> MADYKDDDDKGTDYKDDDDKLEVLFQGPMSLRIDVDTNFPECVVDAGKVTLGTQQRQEMDPRLREKQNEIILRAVCALLNSGGGIIKAEIENKGYNYERHGVGLDVPPIFRSHLDKMQKENHFLIFVKSWNTEAGVPLATLCSNLYHRERTSTDVMDSQEALAFLKCRTQTPTNINVSNSLGPQAAQGSVQYEGNINVSAAALFDRKRLQYLEKLNLPESTHVEFVMFSTDVSHCVKDRLPKCVSAFANTEGGYVFFGVHDETCQVIGCEKEKIDLTSLRASIDGCIKKLPVHHFCTQRPEIKYVLNFLEVHDKGALRGYVCAIKVEKFCCAVFAKVPSSWQVKDNRVRQLPTREWTAWMMEADPDLSRCPEMVLQLSLSSATPRSKPVCIHKNSECLKEQQKRYFPVFSDRVVYTPESLYKELFSQHKGLRDLINTEMRPFSQGILIFSQSWAVDLGLQEKQGVICDALLISQNNTPILYTIFSKWDAGCKGYSMIVAYSLKQKLVNKGGYTGRLCITPLVCVLNSDRKAQSVYSSYLQIYPESYNFMTPQHMEALLQSLVIVLLGFKSFLSEELGSEVLNLLTNKQYELLSKNLRKTRELFVHGLPGSGKTILALRIMEKIRNVFHCEPANILYICENQPLKKLVSFSKKNICQPVTRKTFMKNNFEHIQHIIIDDAQNFRTEDGDWYGKAKFITQTARDGPGVLWIFLDYFQTYHLSCSGLPPPSDQYPREEINRVVRNAGPIANYLQQVMQEARQNPPPNLPPGSLVMLYEPKWAQGVPGNLEIIEDLNLEEILIYVANKCRFLLRNGYSPKDIAVLFTKASEVEKYKDRLLTAMRKRKLSQLHEESDLLLQIGDASDVLTDHIVLDSVCRFSGLERNIVFGINPGVAPPAGAYNLLLCLASRAKRHLYILKASV

The Schlafen family belongs to the interferon-stimulated genes and its members are involved in cell cycle regulation, T cell quiescence, inhibition of viral replication, DNA-repair and tRNA processing. Here, we present the cryo-EM structure of full-length human Schlafen 5 (SLFN5) and the high-resolution crystal structure of the highly conserved N-terminal core domain. SLFN5 binds tRNA as well as single- and double-stranded DNA, suggesting a potential role in transcriptional regulation. The N-terminal Slfn core domain (residues 1–336) is followed by a linker domain (residues 337–552) and a C-terminal helicase/ ATPase domain (residues 553–891).

To gain insights into the structural organization of subgroup III Schlafen proteins, we employed single particle cryo electron microscopy (cryo-EM). The full-length SLFN5 protein was vitrified in the absence of nucleotides. A 3.5 Å cryo-EM density was calculated, giving insights into the overall domain arrangement. A majority of the protein could be resolved (residues 3–684) with exception of the C-terminal ATPase lobe (residues 685–891), which is likely due to its flexibility. The data was acquired in the absence of nucleotides, suggesting that the missing density of the second ATPase lobe could be due to relative flexibility between the lobes. The N-lobe of the Slfn core forms a second large interface with the linker domain, including several hydrophobic (Ile57, Met89, Phe98, Val479, Tyr514, Pro515, Tyr518) and ionic interactions (Asp87 to Arg487). In addition, the loop connecting the Slfn core to the linker domain (residues 335–366) holds the two domains together. The globular linker domain exhibits a mixed α/β topology and connects the Slfn core and the ATPase domain. The highly conserved SWAVDL motif (residues 424–429) seals the hydrophobic core of the linker domain and interacts with the N-terminal lobe of the helicase. The N-terminal helicase lobe is anchored to the linker domain by an α-helix (residues 561–568).>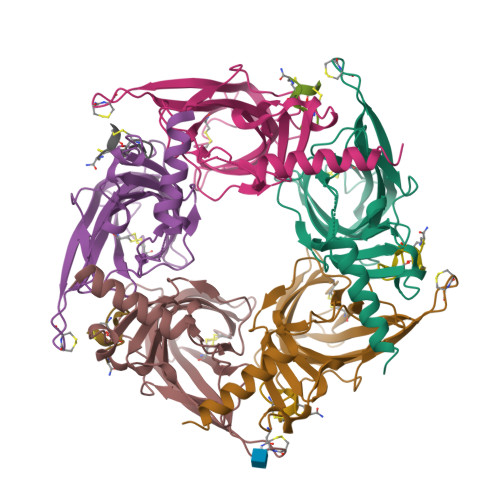[5x]DDDDKLHSQANLMRLKSDLFNRSPMYPGPTKDDPLTVTLGFTLQDIVKADSSTNEVDLVYYEQQRWKLNSLMWDPNEYGNITDFRTSAADIWTPDITAYSSTRPVQVLSPQIAVVTHDGSVMFIPAQRLSFMCDPTGVDSEEGATCAVKFGSWVYSGFEIDLKTDTDQVDLSSYYASSKYEILSATQTRQVQHYSCCPEPYIDVNLVVKFRERR;>[5x]GCCSDPRCAWRC>SLFELGKMILQETGKNPAKSYGAYGCNCGVLGRGKPKDATDRCCYVHKCCYKKLTGCNPKKDRY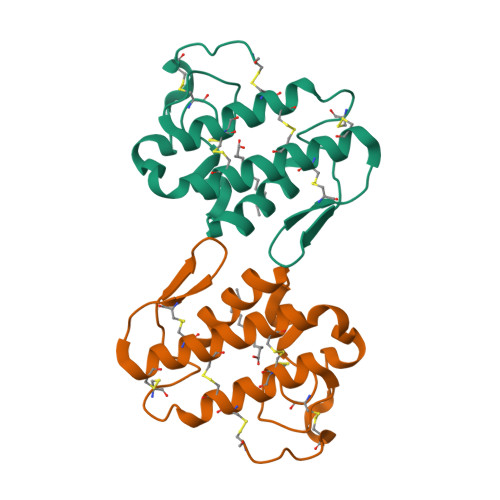SYSWKDKTIVCGENNPCLKELCECDKAVAICLRENLGTYNKKYRYHLKPFCKKADKC[2x]> HHHHHHSSGLVPRGSHDDGKDEEGGSSDGGGGGKTKITLGLFGTAGFEESGLYKEYEKLHPDVDIQQTVVERNENYYPALLNHLTTGSGLQDIQMVEVGNIAEI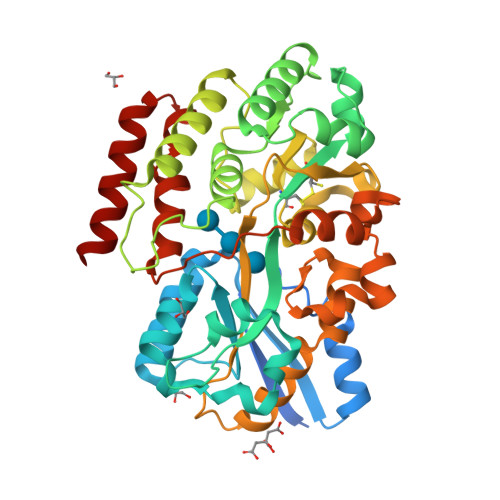VGTQSDKLLDLSKYGKESDYLPWKWSQGSTSGGQTVALGTDVGPMAICYRKDLFEAAGLPSDREEVGKLWTGSWDKFVDAGNQYKKKAPKGTTFLDSPGGLLQAILSSEKDRFYDASGKVIYKTNPAVKSAFDLTAKAAKAGLVGNQTQFQPAWDTTIANSKFAAMSCPPWMLGYIKGKSKPEAAGKWDIAQAPKSGNWGGSFLSVPKNGKNAEEAAKLAAWLTAPEQQAKLFAVQGSFPSTPAAYDSAAVKDAKNDMTGDAPIGTIFAEAAKNIPVQTIGPKDQIIQQGLTDNGVILVTQGKSASDAWKNAVKTIDNALDK>[2x]MLITDTLSPQAFEEALRAKGDFYHIHHPYHIAMHNGDATRKQIQGWVANRFYYQTTIPLKDAAIMANCPDAQTRRKWVQRILDHDGSHGEDGGIEAWLR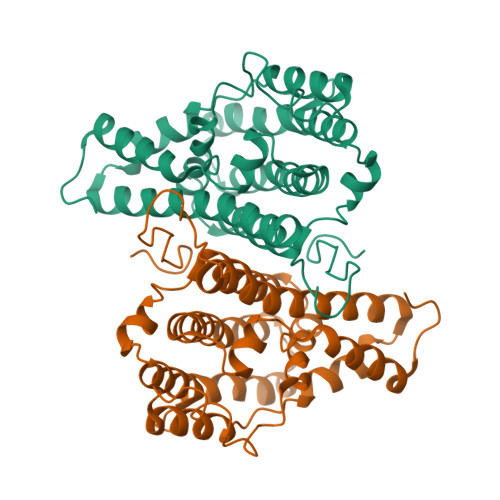LGEAVGLSRDDLLSERHVLPGVRFAVDAYLNFARRACWQEAACSSLTELFAPQIHQSRLDSWPQHYPWIKEEGYFYFRSRLSQANRDVEHGLALAKAYCDSAEKQNRMLEILQFKLDILWSMLDAMTMAYALQRPPYHTVTDKAAWHTTRLVLEHHHHHH> MSAAPVLSITNASVVYPDGISTVTALDSANVEIFPGELVAIVGESGSGKSTLLSIAGFLQE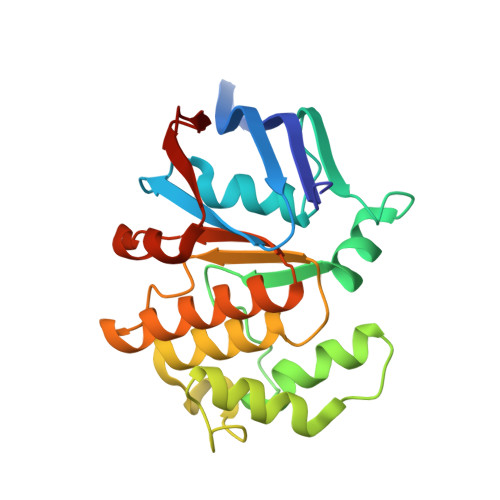PTSGTVTLHGAEGLDATSTRREHIGFVFQQPNLLGSLTAREQLLITDHLRGIKPRKDRADELLARVGLKGLGGRRVAQLSGGQRQRVNIARALMGNPQLLLADEPTSALDARLSKEIVELLRDVTKEFALATLMVTHDRSQLAYADRFVEMADGKALQTA PSEUDOTROPINE | 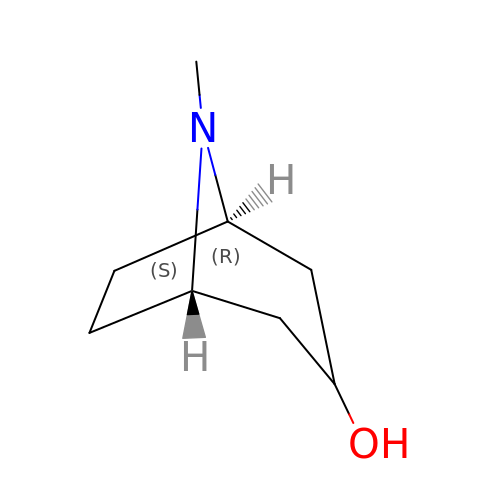C8 H15 N O | CYHOMWAPJJPNMW-RNLVFQAGSA-N> MAVKVEYDLKRLRNIGIAAHIDAGKTTTTERILYYTGRIHKIGEVHEGAATMDFMEQERERGITITAAVTTCFWKDHRINIIDTPGHVDFTIEVERSMRVLDGAIVVFDSSQGVEPQSETVWRQAEKYKVPRIAFANKMDKTGADLWLVIRTMQERLGARPVVMQLPIGREDTFSGIIDVLRMKAYTYGNDLGTDIREIPIPEEYLDQAREYHEKLVEVAADFDENIMLKYLEGEEPTEEELVAAIRKGTIDLKITPVFLGSALKNKGVQLLLDAVVDYLPSPLDIPPIKGTTPEGEVVEIHPDPNGPLAALAFKIMADPYVGRLTFIRVYSGTLTSGSYVYNTTKGRKERVARLLRMHANHREEVEELKAGDLGAVVGLKE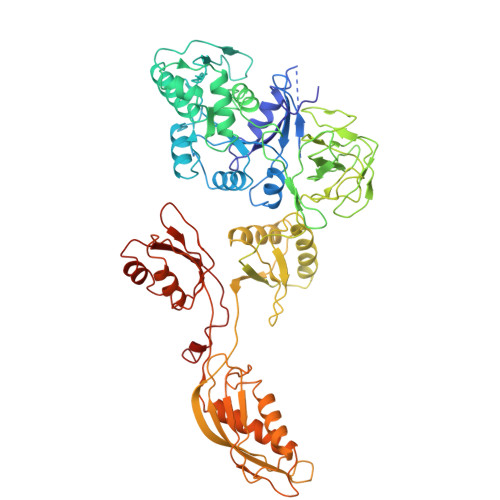TITGDTLVGEDAPRVILESIEVPEPVIDVAIEPKTKADQEKLSQALARLAEEDPTFRVSTHPETGQTIISGMGELHLEIIVDRLKREFKVDANVGKPQVAYRETITKPVDVEGKFIRQTGGRGQYGHVKIKVEPLPRGSGFEFVNAIVGGVIPKEYIPAVQKGIEEAMQSGPLIGFPVVDIKVTLYDGSYAEVDSSEMAFKIAGSMAIKEAVQKGDPVILEPIMRVEVTTPEEYMGDVIGDLNARRGQILGMEPRGNAQVIRAFVPLAEMFGYATDLRSKTQGRGSFVMFFDHYQEVPKQVQEKLIKGQ> SRANDAPIVLLHGFTGWGREEMFGFKYWGGVRGDIEQWLNDNGYRTYTLAVGPLSSNWDRACEAYAQLVGGTVDYGAAHAAKHGHARFGRTYPGLLPELKRGGRIHIIAHSQGGQTARMLVSLLENGSQEEREYAKAHNVSLSPLFEGGHHFVLSVTTIATPHDGTTLVNMVDFTDRFFDLQKFVLKAAAVASNVPYTSQVYDF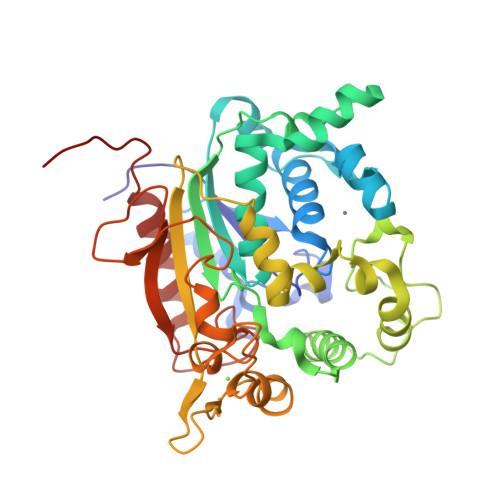KLDQWGLRRQPGESFDQYFERLKRSPVWTSTDTARYDLSVPGAEKLNQWVKASPNTYYLSFATERTYRGALTGNYYPELGMNAFSAVVCAPFLGSYRNATLGIDDRWLENDGIVNAFSMNGPKRGSTDRIVPYDGTIKKGVWNDMGTYNVDHFEVIGVDPNPLFDIRAFYLRLAEQLASLQPHHHHHH> UXCUCCUAGUACGAGAGGACCGG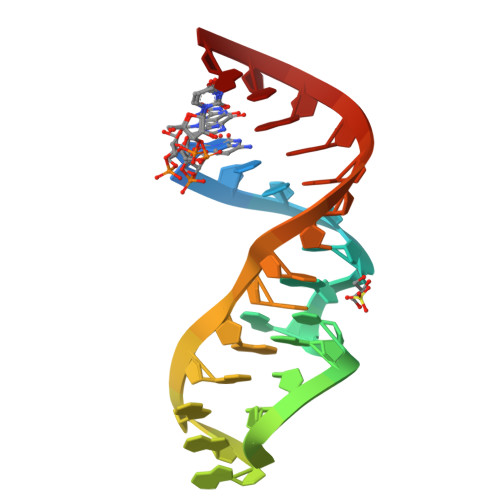AGUG> MNDPNLFVALYDFVASGDNTLSITKGE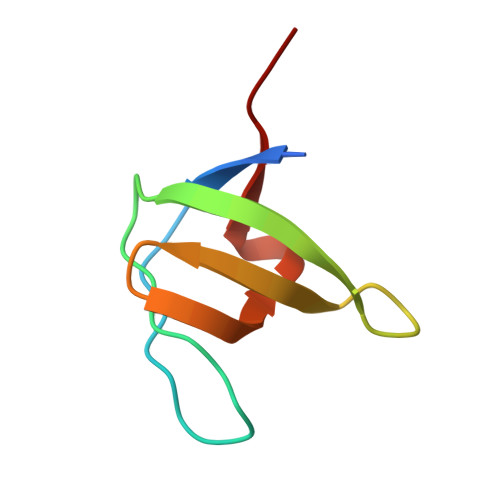KLRVLGYNHNGEWCEAQTKNGQGWVPSNYITPVNS>[2x]MAHHHHHHMDSLKKIVAYKAVDEY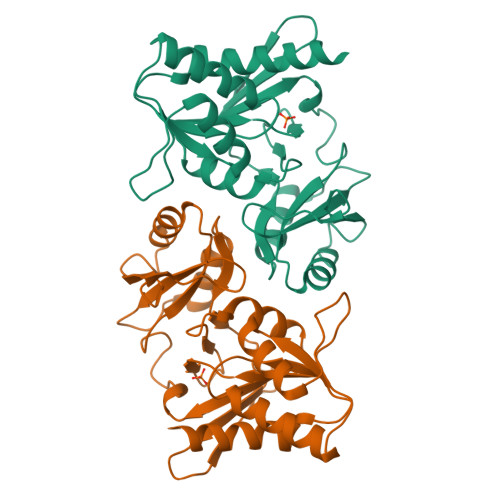VQSNMTIGLGTGSTVFYVLERIDNLLKSGKLKDVVCIPTSIDTELKARKLGIPLTTLEKHSNIDITIDGTDEIDLNLNLIKGRGGALVREKLVASSSSLLIIIGDESKLCTNGLGMTGAVPIEILTFGYEKIIENLLKIYTLKGCTYKIRKRNGEIFITDNKNYIVDFFFTEPIQDLLETCTRIKMTTGVVDHGIFVNMTNVALISKHDGTVLTLNKKYE1,3,2-DIOXABOROLAN-2-OL | C2 H5 B O3 | 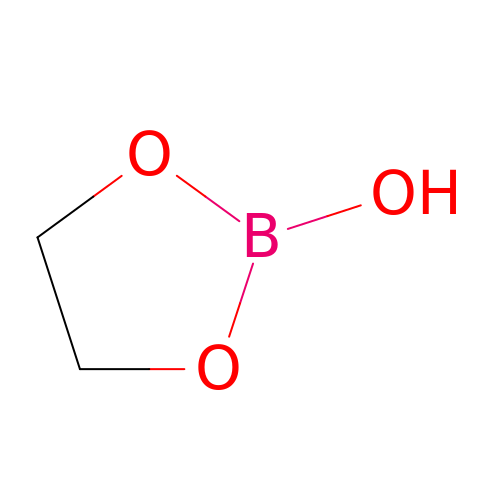ZBEDLGKSWBORBS-UHFFFAOYSA-N>APIKVGINGFGRIGRMVFQAICDQGLIGTEIDVVAVVDMSTNAEYFAYQMKHDTVHGRPKYTVEAVKSSPSVETADVLVVNGHRIKCVKAQRNPADLPWGKLGVDYVIESTGLFTD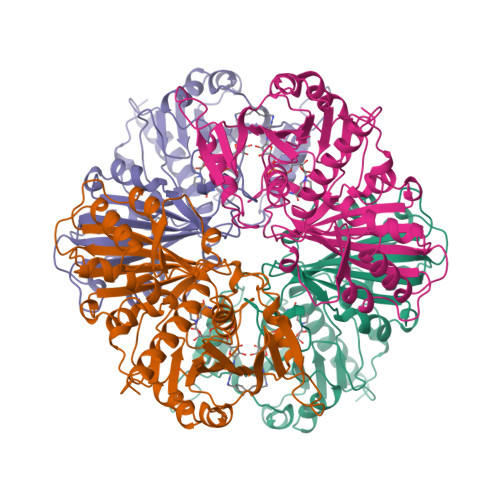KLKAEGHIKGGAKKVVISAPASGGAKTIVMGVNQHEYSPASHHVVSNASCTTNCLAPIVHVLTKENFGIETGLMTTIHSYTATQKTVDGVSLKDWRGGRAAAVNIIPSTTGAAKAVGMVIPSTKGKLTGMSFRVPTPDVSVVDLTFRATRDTSIQEIDKAIKKAAQTYMKGILGFTDEELVSADFINDNRSSVYDSKATLQNNLPGEKRFFKVVSWYDNEWAYSHRVVDLVRYMAAKDAASS[4x]> KGTFKDYVRDRADLNKDK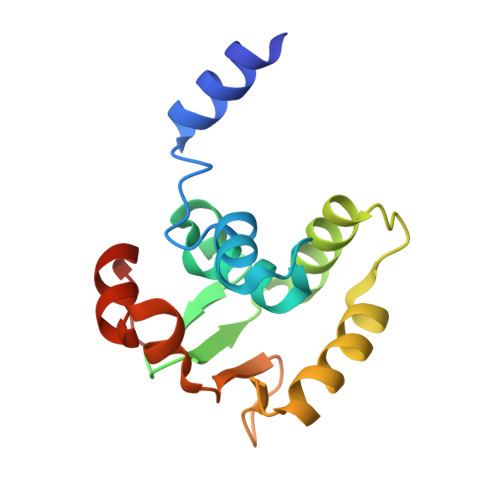PVIPAAALAGYTGSGPIQLWQFLLELLTDKSCQSFISWTGDGWEFKLSDPDEVARRWGKRKNKPKMNYEKLSRGLRYYYDKNIIHKTAGKRYVYRFVCDLQSLLGYTPEELHAMLDVKPDAD>QAQITGRPEWIWLALGTALMGLGTLYFLVKGMGVSDPDAKKFYAIATLVPAIAFTMYLSMLLGYGLTMVPFGGEQNPIYWARYADWLFTTPLLLLDLALLVDADQGTILALVGADGIMIGTGLVGALTKVYSYRFVWWAISTAAMLYILYVLFFGFTSKAESMRPEVASTFKVLRNVTVVLWSAYPVVWLIGSEGAGIVPLNIETLLFMVLDVSAKVGFGLILLRSRAIFGEAEAPEPSA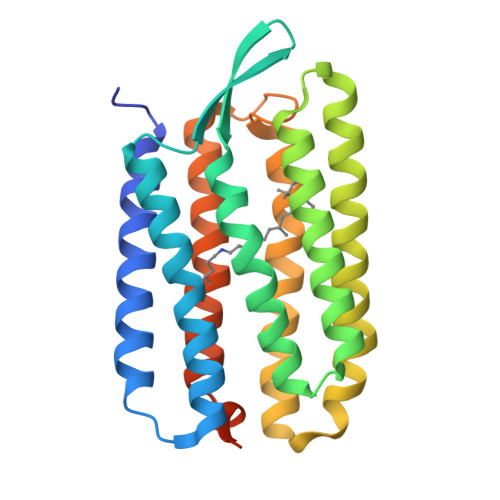GDGAAATSD[2x]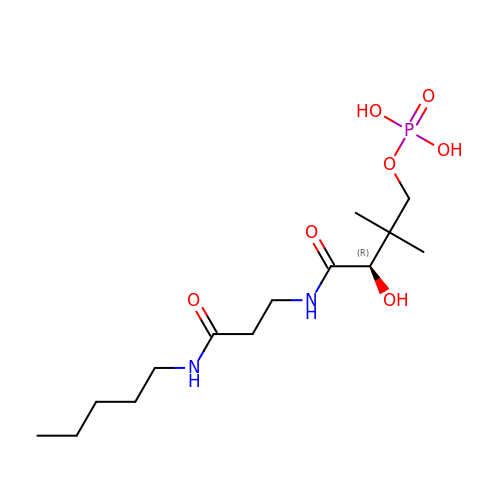N~3~-[(2R)-2-hydroxy-3,3-dimethyl-4-(phosphonooxy)butanoyl]-N-pentyl-beta-alaninamide | C14 H29 N2 O7 P | YNPRWOBMMGRKHD-LBPRGKRZSA-N>TDLIQRPRRLRKSPAL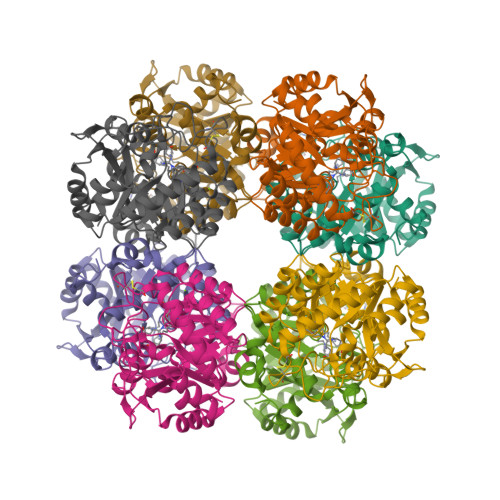RAMFEETTLSLNDLVLPIFVEEEIDDYKAVEAMPGVMRIPEKHLAREIERIANAGIRSVMTFGISHHTDETGSDAWREDGLVARMSRICKQTVPEMIVMSDTCFCEYTSHGHCGVLCEHGVDNDATLENLGKQAVVAAAAGADFIAPSAAMDGQVQAIRQALDAAGFKDTAIMSYSTKFASSFYGPFREAAGSALKGDRKSYQMNPMNRREAIRESLLDEAQGADCLMVKPAGAYLDIVRELRERTELPIGAYQVSGEYAMIKFAALAGAIDEEKVVLESLGSIKRAGADLIFSYFALDLAEKKILR[2x]>[5x]TDVAKTLEELATERGMRMTEQRRVIARILEDSEDHPDVEELYRRSVKVDAKISISTVYR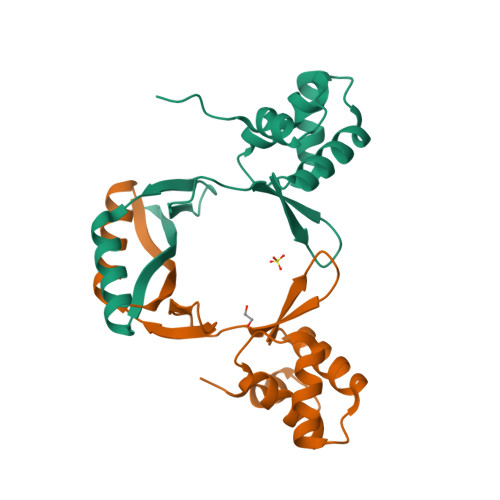TVKLFEDAGIIARHDFRDGRSRYETVPEEHHDHLIDLKTGTVIEFRSPEIEALQERIAREHGFRLVDHRLELYGVPLKKEDL WW domains organize molecular assemblies by binding to short, proline rich peptide motifs each with ~4–6 residues. The type I WW domains bind to a consensus ‘PPxY’ motif (where P is proline, x is any amino acid and Y is tyrosine, also known as PY-motif) with very modest affinities (with Kd in the range of a few to a few tens of µM). To achieve this goal, we determined the high resolustion structures of 7 representative WW tandem/target complexes, and measured the binding constants of >100 WW domain tandems or isolated WW domains binding to known or previously unknown targets. In this study, we discovered that WW tandems, but not individual WW domains, can bind to target proteins with extremely high affinity and with very high sequence specificity.

By sequence alignment of WW tandems, including those from KIBRA, MAGIs, YAP, SAV1, WWOX, ITCH WW12 and ITCH WW34, we found that MAGI2 and MAGI3 WW tandems have striking similarities to KIBRA WW tandem both in the inter-domain linker (23 aa in MAGI2 and MAGI3 vs 24 aa in KIBRA and with ~60% sequence similarity) and in the C-terminal helix regions. We further found that MAGI2 and MAGI3 WW tandems bind to Dendrin PY23 with extremely high affinities (Kd values of ~2.3 and~3.6 nM), further supporting the conclusion that MAGI2, MAGI3 and KIBRA WW tandems share a high similarity in target bindings. We solved the crystal structure of MAGI2 WW tandem in complex with Dendrin PY23 at the 1.65 Å resolution. A structural comparison of the MAGI2 WW tandem in complex with Dendrin with those of the KIBRA WW tandem in complex with various ligands shown in Figure 2 showed that the overall structures of KIBRA and MAGI2 WW tandems in these complexes are similar to each other (RMSD values of 2.3–2.7 Å for the Cα atoms). Notably, the extensive interactions between the inter-domain linker and the C-terminal helix stabilize the supramodular structure of the MAGI2 WW tandem, and the Dendrin PY23 binds to the MAGI2 WW tandem following almost the exactly same detailed interactions as those observed in the KIBRA WW12/Dendrin PY23 complex. In the WW tandem structures of KIBRA and MAGI2, a hydrophobic residue from WW1 (I35 in KIBRA and L330 in MAGI2) inserts into a hydrophobic pocket formed by WW2 domain and the inter-domain linker. Indeed, the I35D substitution weakened KIBRA’s binding to PTPN14 PY12 by ~50 fold, and the L330D mutation decreased MAGI2’s binding to Dendrin PY23 by ~57 fold. The extensive interactions between the inter-domain linker and the C-terminal helix couples the two WW domain into a structural supramodule in these WW tandems, thus providing a structural and thermodynamic basis for highly synergistic bindings to target proteins.

>GPGSEFEENEDSDPLPDNWEMAYTEKGEVYFIDHNTKTTSWLDPRLAKKAKPPEECKENELPYGWEKIDDPIYGTYYVDHINRRTQFENPVLEAKRKLQQHN[2x];>GPGSDRPPPYVAPPSYEG[2x]>MSQTHKHAIPANIADRCLINPEQYETKYKQSINDPDTFWGEQGKILDWITPYQKVKNTSFAPGNVSIKWYEDGTLNLAANCLDRHLQENGDRTAIIWEGDDTSQSKHISYRELHRDVCRFANTLLDLGIKKGDVVAIYMPMVPEAAVAMLACARIGAVHSVIFGGFSPEAVAGCIIDSSSRLVITADEGVRAGRSIPLKKNVDDALKNPNVTSVEHVIVLKRTGSDIDWQEGRDLWWRDLIEKASPEHQPEAMNAEDPLFILYTSGSTGKPKGVLHTTGGYLVYAATTFKYVFDYHPGDIYWCTADVGWVTGHSYLLYGPLACGATTLMFEGVPNWPTPARMCQVVDKHQVNILYTAPTAIRALMAEGDKAIEGTDRSSLRILGSVGEPINPEAWEWYWKKIGKEKCPVVDTWWQTETGGFMITPLPGAIELKAGSATRPFFGVQPALVDNEGHPQEGATEGNLVITDSWPGQARTLFGDHERFEQTYFSTFKNMYFSGDGARRDEDGYYWITGRVDDVLNVSGHRLGTAEIESALVAHPKIAEAAVVGIPHAIKGQAIYAYVTLNHGEEPSPELYAEVRNWV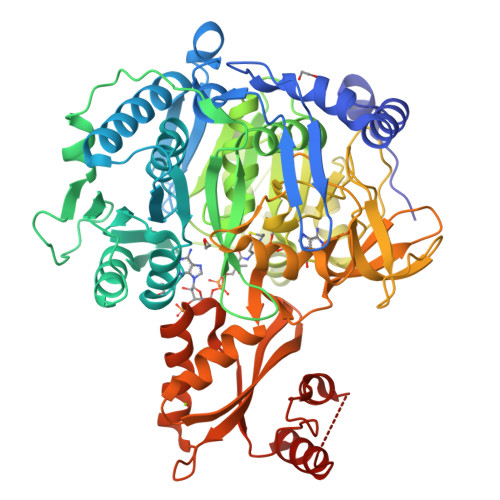RKEIGPLATPDVLHWTDSLPKTRSGKIMRRILRKIAAGDTSNLGDTSTLADPGVVEKLLEEKQAIAMPS[2x]> AAGHVNIAEAVQQLNHTIVNAAHELHETLGLPTPDEALNLLTEQANAF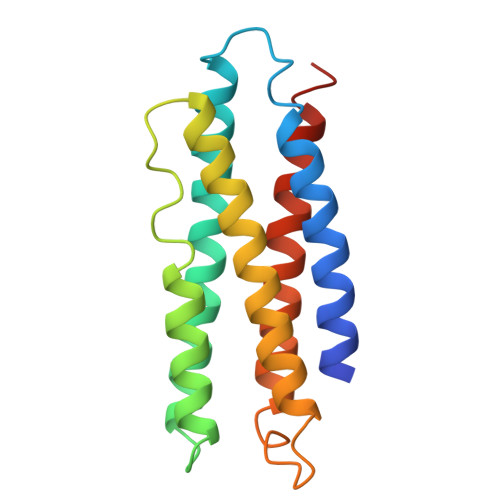KTKIAEVTTSLKQEAEKHQGSVAEQLNAFARNLNNSIHDAATSLNLQDQLNSLQSALTNVGHQWQDIATKTQASAQEAWAPVQSALQEAAEKTKEAAANLQNSIQSAVQKPAN>MATSGFKHLVVVKFKEDAKVDEI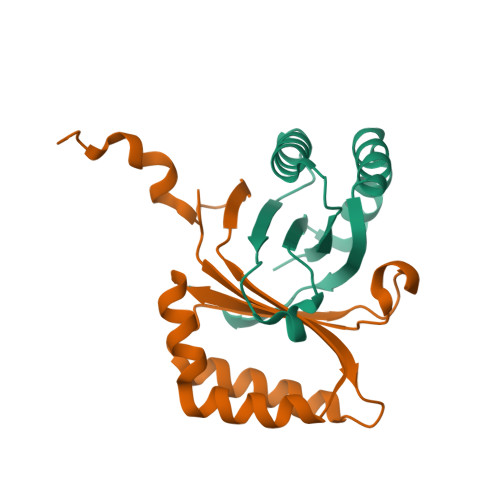LKGLENLVSQIDSVKSFEWGEDNESHEMLRQGFTHAFSMTFENKDAYVSFTGHPLHVEFSAAFTAVIDKIVVMDFTVAAVKSPVVVAPAAALEWSHPQFEK[2x]>MAHHHHHHGGSEPFYITTAIAYP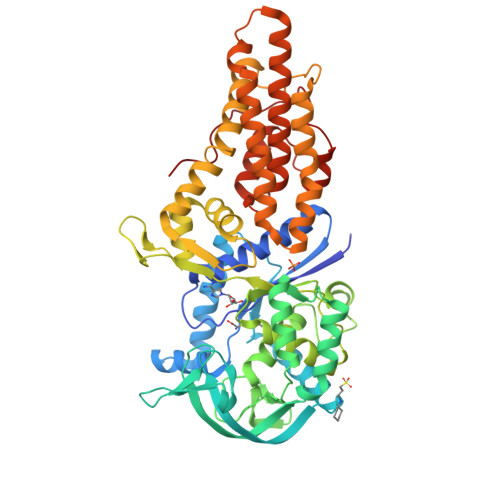NGVPHIGHAYEYIATDAIARFKRLDGYDVRYLTGTDVHGQKMAETAAKEGIPAAELARRNSDVFQRLQEKLNISFDRFIRTSDADHYEASKAIWKRMADAGDIYLDAYKGWYSIRDERFFTENETTEQPDGTRIATETGAPVTWTEEQTYFFRLSAYTDRLLALYEEHPEFIGPDARRNEIVSFVSGGLKDLSISRTTFDWGVPVPDHPDHVMYVWVDALTNYLTGVGFPDTESESFRRYWPADLHMIGKDIIRFHTVYWPAFLMSAGLPLPKRIFAHGWLLNRGEKMSKSIGNVVDPVNLVDTFGLDQVRYFLLREVPFGQDGSYNEDAIIGRVNADLANELGNLAQRSLSMVAKNLGAAVPDPGEFTDEDTALLAAADALLERVREHFDVPAMHLALEAIWSVLGAANRYFSAQEPWVLRKSDAAEDQQRFRTVLYTTLEVVRIASLLLQPVMPESTAKLLDLLGQPTDERDFSAIANRIKPGTSLPAPSGIFPRYQND[3x]>[2x]CC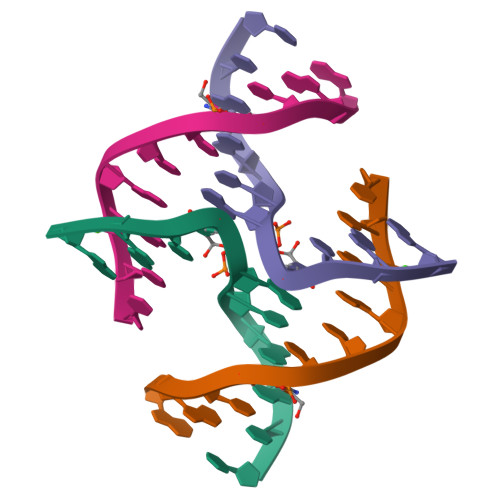GGCGXCGG> MSEKKEARVVINDLLAEQYANAFKAKEEGRPVGWSTSVFPQELAEVFDLNVLYPENQAAGVAAKKGSLELCEIAESKGYSIDLCAYARTNFGLLENGGCEALDMPAPDFLLCCNNICNQVIKWYENISRELDIPLIMIDTTFNNEDEVTQSRIDYIKAQFEEAIKQLEIISGKKFDPKKFEEVMKISAENG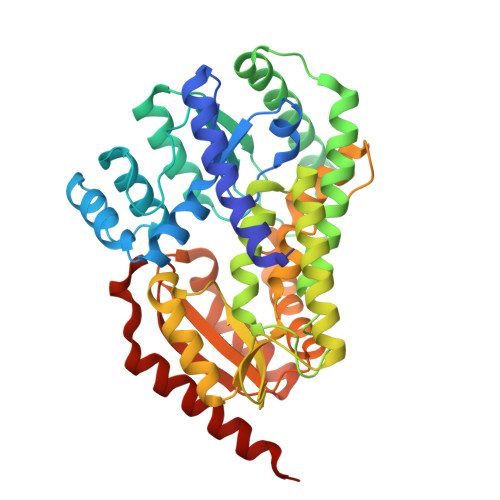RLWKYSMSLPADSSPSPMNGFDLFTYMAVIVCARGKKETTEAFKLLIEELEDNMKTGKSSFRGEEKYRIMMEGIPCWPYIGYKMKTLAKFGVNMTGSVYPHAWALQYEVNDLDGMAVAYSTMFNNVNLDRMTKYRVDSLVEGKCDGAFYHMNRSCKLMSLIQYEMQRRAAEETGLPYAGFDGDQADPRAFTNAQFETRIQGLVEVMEERKKLNRGEI>[2x]GSSMSRAAQLLPGTWQVTMTNEDGQTSQGQWHFQPRSPYTMDIVAQGTISDGRPIVGYGKATVKTPDTLDIDITYPSLGNIKAQGQITM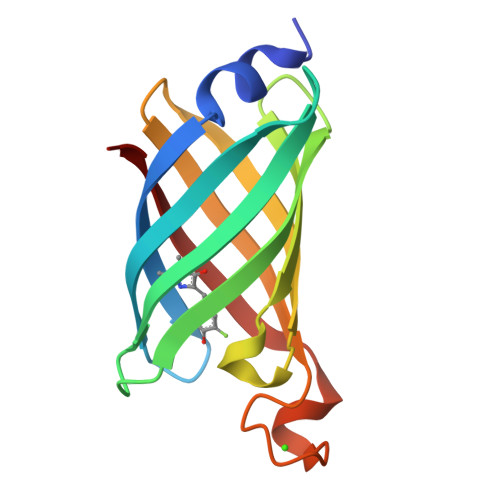DSPTQFKWDAHYKGDKDGDGYISAAEAAAQGLTGTLQRQE L-GAMMA-GLUTAMYL-S-OCTYL-D-CYSTEINYLGLYCINE | C18 H33 N3 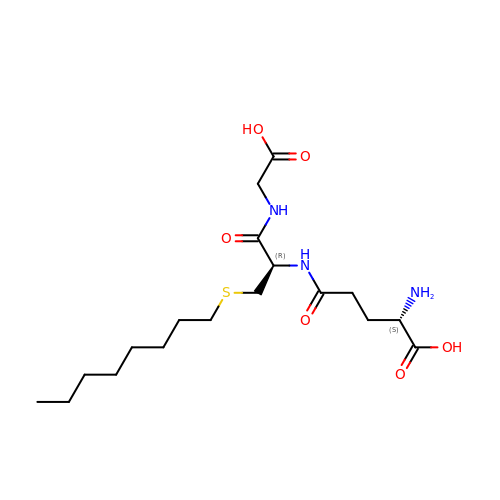O6 S | MJWCZWAVSJZQNL-KBPBESRZSA-N> GMDFLTSTLLSGILYDGFKNGVAITTGFLKEK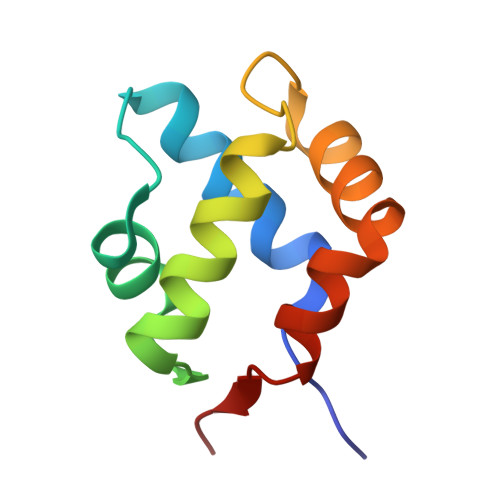LHGWIVDDTLLETLAYKVNTLELKDYGEHVIERKLNESSEIQQILKLIQPEQ>[2x]AVPFVEDWDLVQTLGEGAYGEVQLAVNRVTEEAVAVKIVDMKRAVDCPENIKKEICINKMLNHENVVKFYGHRREGNIQYLFLEYCSGGELFDRIEPDIGMPEPDAQRFFHQLMAGVVYLHGIGITHRDIKPENLLLD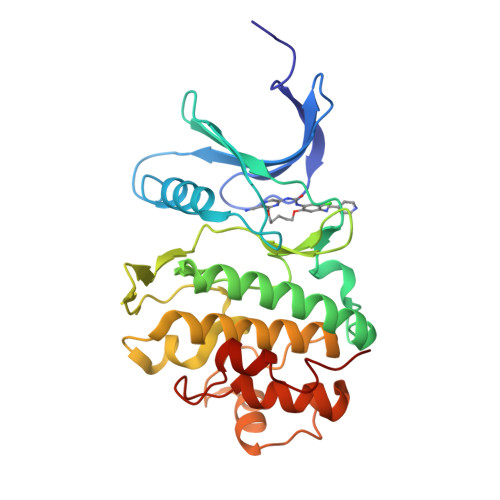ERDNLKISDFGLATVFRYNNRERLLNKMCGTLPYVAPELLKRREFHAEPVDVWSCGIVLTAMLAGELPWDQPSDSCQEYSDWKEKKTYLNPWKKIDSAPLALLHKILVENPSARITIPDIKKDRWYNKPL> MSEDTIIGFLGQPVTLPCHYLSWSQSRNSMCWGKGSCPNSKCNAELLRTDGTRIISRKSTKYTLLGKVQFGEVSLTISNTNRGDSGVYCCRIEVPGW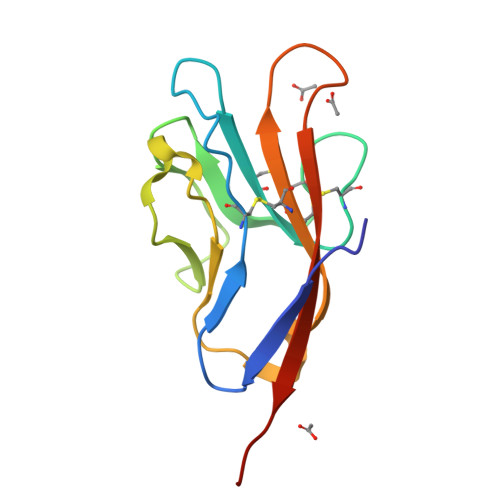FNDVKKNVRLELRRALVPR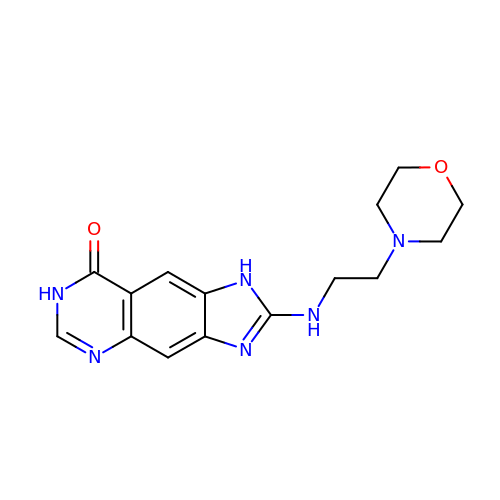2-{[2-(4-Morpholinyl)ethyl]amino}-1,7-dihydro-8H-imidazo[4,5-g]quinazolin-8-one | C15 H18 N6 O2 | IQPSZZDLHUVVGO-UHFFFAOYSA-N> GPAE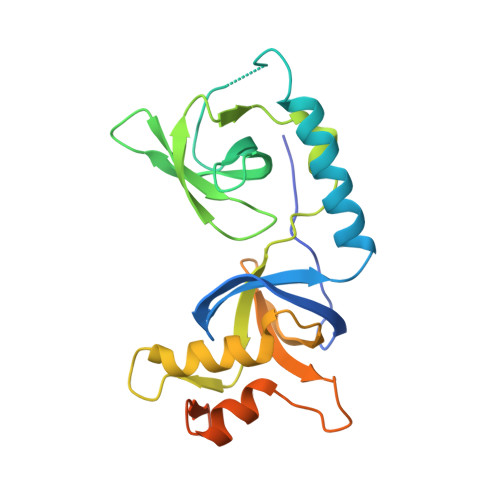ALEWTWVEFTVDETVDVVVCMMYSPGEFYCHFLKDDALEKLDDLNQSLADYCAQKPPNGFKAEIGRPCCAFFSGDGNWYRALVKEILPSGNVKVHFVDYGNVEEVTTDQLQAILPQFLLLPFQGMQCWLVDIQPPNKHWTKEATARFQACVVGLKLQARVVEITANGVGVELTDLSTPYPKIISDVLIREQLVLRCGSPQDSLMSRPANQHKQIDSHRVQAS>M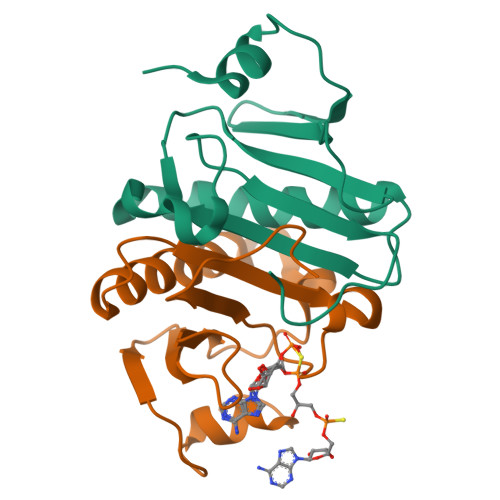ADEIAKAQVARPGGDTIFGKIIRKEIPAKIIFEDDRCLAFHDISPQAPTHFLVIPKKHISQISVAEDDDESLLGHLMIVGKKCAADLGLNKGYRMVVNEGSDGGQSVYHVHLHVLGGRQMHWPPG[4x]> 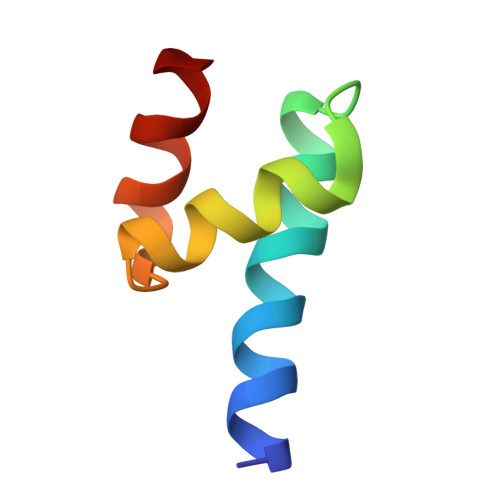LSELEDLKDAKLQTLKELFPQRSDNDLLKLIESTSTMDGAIAAALLMF>MGSDKIHHHHHHMQTFLKGKRVGYWLSEKKIKKLNFQAFAELCRKRGMEVVQLNLSRPIEEQGPLDVIIHKLTDVILEADQNDSQSLELVHRFQEYIDAHPETIVLDPLPAIRTLLDRSKSYELIRKIEAYMEDDRICSPPFMELTSLCGDDTMRLLEKNGLTFPFICKTRVAHGTNSHEMAIVFNQEGLNAIQPPCVVQNFINHNAVLYKVFVVGESYTVVQRPSLKNFSAGTSDRESIFFNSHNVSKPESSSVLTELDKIEGVFERPSDEVIRELS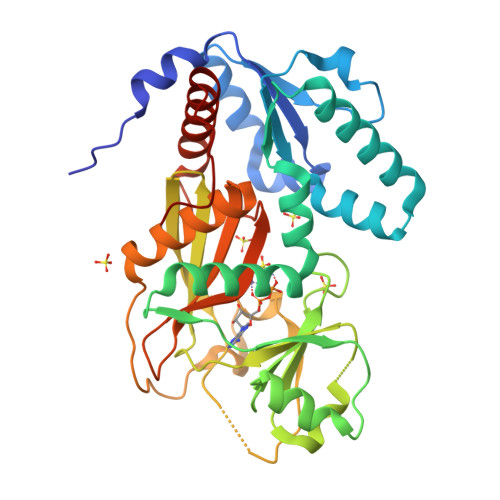RALRQALGVSLFGIDIIINNQTGQHAVIDINAFPGYEGVSEFFTDLLNHIATVLQGQSTAMAATGDVAL[2x]> MREQRKGEDGYNWRKYGQKQVKGSENPRSYYKCTFPNCPTKKKVERSLEGQITEIVYKGSHNHPKPLEHH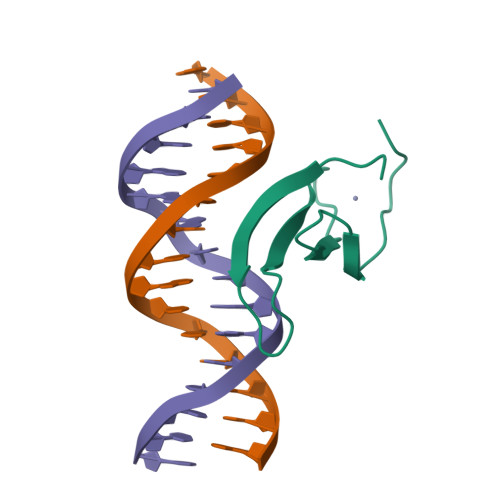HHHH> SMHLICQSGDVLSARYEIVDTLGEGAFGKVVECIDHKAGGRHVAVKIVKNVDRYCEAARSEIQVLEHLNTTDPNSTFRCVQMLEWFEHHGHICIVFELLGLSTYDFIKENGFLPFRLDHIRKMAYQICKSVNFLHSNKLTHTDLKPENILFVQSDYTEAYNPKIKRDERTLINPDIKVVDFGSATYDDEHHSTLVSTRHYRAPEVILALGWSQPCDVWSIGCILIEYYLGFTVFPTHDSKEHLAMMERILGPLPKHMIQKTRKRKYFHHDRLDWDEHSSAGRYVSRACKPLKEFMLSQDVEHERLFDLIQKMLEYDPAKRITLREALKHPFFDLLKKSI

Extracellular signal-regulated kinase 3 (ERK3) is a poorly studied member of the mitogen-activated protein kinase (MAPK) family. Similar to ERK4, ERK7, and NLK, ERK3 is classified as an atypical MAPK. Despite potentially important functions in cellular processes and tumorigenesis, no ERK3-selective inhibitors have been published that could be used as tools to elucidate the roles of this kinase in normal and pathological signalling processes. To contribute to recent global research efforts on untargeted human proteins, we present the crystal structure as well as the discovery of inhibitors of ERK3, providing a foundation for the development of selective inhibitors for this poorly-studied, atypical MAPK kinase.

In order to provide structural insights into inhibitor binding, we attempted to determine the complex structure of ERK3 and inhibitors. Unfortunately, we did not succeed in obtaining crystals of any complexes, either by co-crystallization or soaking. Therefore, we determined the structure of CAF052 in complex with CDC-like kinase 1 (CLK1), which belongs to the same kinase group (CMGC) as ERK3, and performed structural comparison. In CLK1, CAF052 adopted a typical type-I binding mode, utilizing its 2-aminopyrimidine core for the interactions with the backbone of the hinge residue L244. Structural superimposition demonstrated that although sharing a low-sequent identity the binding mode of the inhibitor, as well as the contacts with the hinge region observed in CLK1, could most likely be maintained in ERK3. Nevertheless, other interactions observed in CLK1 might differ in ERK3 due to amino acid variations. This included the contact between the inhibitor piperazine and the αD D250 in CLK1, which might likely be absent in ERK3 harbouring N117 at this position. In this binding mode, the pyrazolopyridazine group was expected to still bind within the back pocket of ERK3 and form a contact with the β3 catalytic lysine. Nonetheless, other interactions engaged by this moiety were presumably different, due to the substitutions of a F241 gatekeeper and V324 in CLK1 for Q108 and G171, respectively, in ERK3. This structural comparison therefore suggests that ERK3 likely shares similar mechanisms for accommodating inhibitors to that of other kinases, enabling binding of various inhibitors that are developed for protein kinases from diverse families.>GEKKQTSEFPDWAWADFQRPE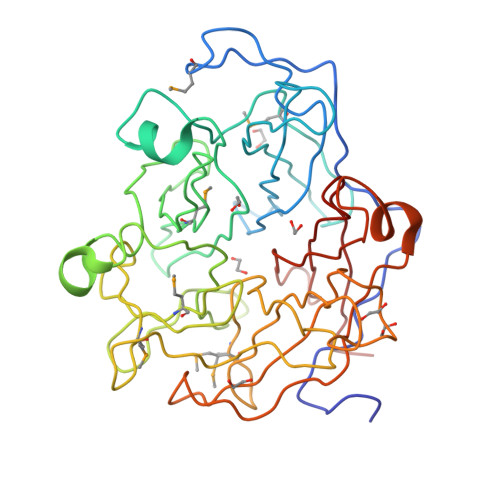GINPIVSPDTTTVFYCPMRQDSVAWESSDTFNPAATIYDGKVVVLYRAEDNSAVGIGSRTSRLGYAYSDDGLHFNRMTVPVFYPADDNQKELEWPGGCEDPRVAVTEDGLYVMLYTQWNRKQARLAVATSRDLQIWEKYGPAFAKAYGGRFFDEFSKSASIVTKLVDGKQVIAKIDGKYWMYWGEKFVNVATSTDLINWEPMLDEKGDFLKVITPREGKFDSDLTECGPPAIMTDKGILLLYNGKNKSGAEGDTLYTANSYCAGQALFDAKDPTKLIDRLDKPFYIPESDFEKSGQYPAGTVFIEGLVFHNQKWYLYYGCADSRVAVAVYDPFKK[4x]>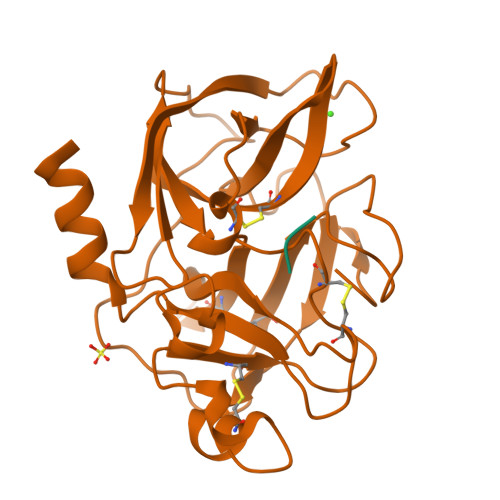 VVGGTEAQRNSWPSQISLQYRSGSSWAHTCGGTLIRQNWVMTAAHCVDRELTFRVVVGEHNLNQNNGTEQYVGVQKIVVHPYWNTDDVAAGYDIALLRLAQSVTLNSYVQLGVLPRAGTILANNSPCYITGWGLTRTNGQLAQTLQQAYLPTVDYAICSSSSYWGSTVKNSMVCAGGDGVRSGCQGDSGGPLHCLVNGQYAVHGVTSFVSRLGCNVTRKPTVFTRVSAYISWINNVIASN;> MFLE>[2x]MDEGMWLMQQLGRKYAQMKERGLKMKEYDLYNPNGTSLKDAVVLFDGGCTGEVVSDRGLVLTNHHCGYDMIQAHSTLEHNYLENGFWAMREADELPNKDISVVFIDKIEDVTDYVKKELKAIKDPNSMDYLSPKYLQKLADKKAGKNFSAKNPGLSVEIKAFYGGNLYLMFTKKTYTDVRLVGAPPSSIGKFGADTDNWIWPRHTGDFSIFRIYADKNGNPAPYSEDNVPLKPKRFFNISLGG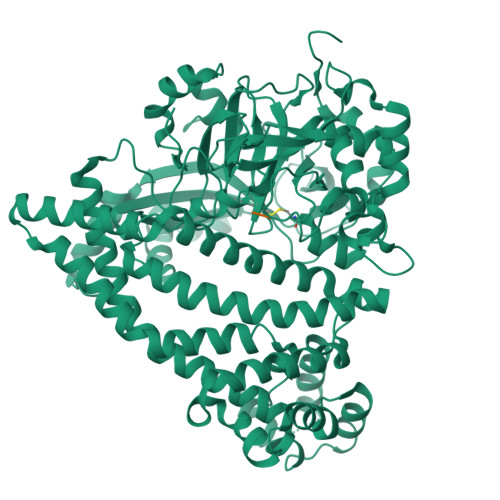VQENDYAMIMGFPGTTHRYFTASEVDEWKSIDNDIRIRMRDIRQGVMLREMLADPQIKIMYSAKYAASQNAYKRAIGANWAIKTRGLRQNKQAMQDRLIAWGAKQGTPRYEEAVHEIDATVAKRADLRRRYWMIEEGIIRGIEFARSPIPTEDETKALQGNDASARKEAIDKIRTRYSKFANKDYSAEVDKKVAVAMLTEYLKEIPYENLPLHLRLVKDRFAGDVQAYVDDIFARSVFGSEAQFDAFAAVPSVEKLAEDPMVLFASSVFDEYRKLYNELRPYDDPILRAQRTYIAGLLEMDGDQDQFPDANLTLRFTYGQVKGYSPRDNVYYGHQTTLDGVMEKEDPDNWEFVVDPKLKAVYERKDFGRYADRSGRMPVAFCATTHTTGGNSGSPVMNANGELIGLNFDRNWEGVGGDIQYLADYQRSIIVDIRYVLLVIDKVGGCQRLLDEMNIVPAHHHHHH;>RD[2x]(3-bromo-2-oxo-propoxy)phosphonic acid 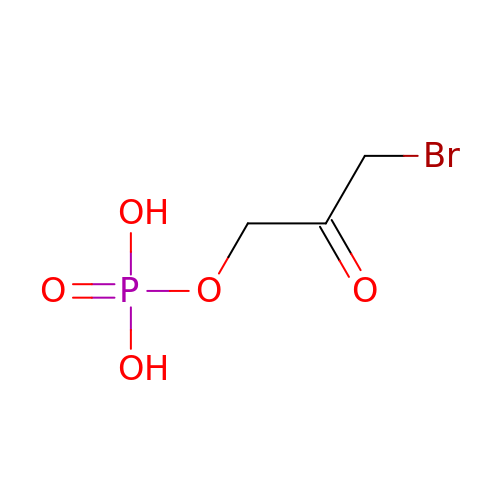| C3 H6 Br O5 P | QXVSTTOPPFAZGJ-UHFFFAOYSA-N N-(4-nitrophenyl)cyclopropanecarboxamide | C10 H10 N2 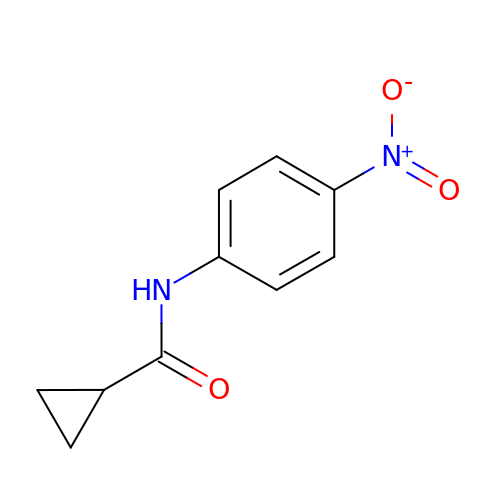O3 | PXCMXAOVWGQBSS-UHFFFAOYSA-N> MSLLPTAPVRIDADLYDDLANPARQSLYPRDSRGFIRIDISLRAYWHTLFDTCPRLLELSGPSGGAIFLPFMAWARENNLAFDWSFFLWVYVWLQQSEFRERLDEDQLLPVMTASATRWLMIDRDIDACQIVLGSRSLAGAAV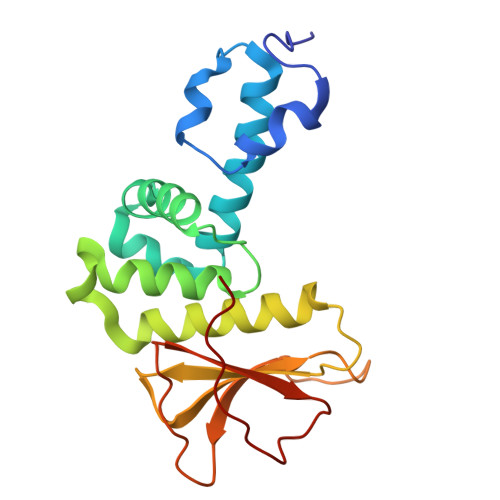VGAKIDSIHCRLEQVQQVAFAAPLPLPDGEFGYFLTPGFEIDHFPGWRPLPR>[2x]MGSDKIHHHHHHMFRGVGTAIVTPFKNGELDLESYERLVRYQLENGVNALIVLGTTGESPTVNEDEREKLVSRTLEIVDGKIPVIVGAGTNSTEKTLKLVKQAEKLGANGVLVVTPYYNKPTQEGLYQHYKYISERTDLGIVVYNVPGRTGVNVLPETAARIAADLKNVVGIKEANPDIDQIDRTVSLTKQARSDFMVWSGNDDRTFYLLCAGGDGV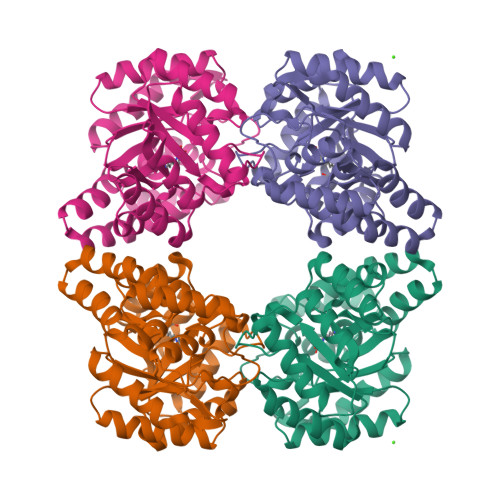ISVVSNVAPKQMVELCAEYFSGNLEKSREVHRKLRPLMKALFVETNPIPVKAALNLMGFIENELRLPLVPASEKTVELLRNVLKESGLL> TQVHMLYINAEVNGISIKAFVDSGAQTTIMSKKCAEKCNLVRLIDYRFSGIAQGVGTSKIVGKIHVAQMKIGNSFFPFSITVLEESHVDFLFGLDLLKRYQCCIDLHQNALIIGDEKVQFLSESEINS

Ddi1 is a multidomain protein that belongs to the ubiquitin receptor family of proteins. The Ddi1 proteins contain a highly conserved retroviral protease (RVP)-like domain along with other domains. The crystal structures of the RVP domains of Ddi1 from T. gondii and C. hominis were determined; they form homodimers similar to those observed in HIV protease and the reported structures of the same domain from Saccharomyces cerevisiae, Leishmania major and humans. The ubiquitin receptor family of proteins bind to ubiquitinated substrates through the UBA domain and deliver the substrates to the proteasome by interacting with the regulatory subunit of the 26S proteasome through the UBL domain.

The structure of CrypDdi1-RVP was determined by molecular replacement using the ToxoDdi1-RVP structure as the search model which has 61% sequence identity with ToxoDdi1-RVP. The solution had one molecule in the ASU with TFZ and LLG of 29 and 899, respectively, in the space group H32. The electron density corresponding to the flap region was missing. The dimer could be generated upon application of the crystallographic 2-fold symmetry. Similarly in the CrypDdi1-RVP structure, the side chains of residues Met203, Tyr205, Phe218, Ala223, Ile227, Ile258, Thr279, Leu281, Val286 and Leu289 form a hydrophobic binding cavity. The binding cavity in the ToxoDdi1-RVP structure has a width of ∼27 ​Å (distance between the Cα atoms of Asn379 residues of the two subunits of the dimer), while in the CrypDdi1-RVP structure, the cavity width is ∼22.5 ​Å (distance between the Cα atoms of Ser284 of the two subunits). The cavity in ToxoDdi1-RVP is larger than that formed in HIV protease which has a width of ∼19–22 ​Å in the open form, while the size of the cavity in CrypDdi1-RVP is comparable to that of HIV protease. Of all the inhibitors tested, nelfinavir showed binding to ToxoDdi1-RVP with a Kd of 237.6 ​± ​6.3 ​μM and saquinavir showed binding to CrypDdi1-RVP with a Kd of 242.1 ​± ​3 ​μM. Saquinavir docked to CrypDdi1-RVP with a binding energy of −6.5 ​kcal/mol in a similar manner as observed in the crystal structure of the complex of HIV protease with saquinavir. While the presence of HDD and the similarities in the structures and the active site architecture suggest that ToxoDdi1-RVP may have the capability to cleave ubiquitin and the substrates upon polyubiquitination similar to the yeastDdi1, in the case of CrypDdi1-RVP as the HDD domain is missing, the triggering mechanism has to be different and is yet to be investigated.> GPHMGAKWHLGIRSQSKPNDIMLEVYRAMKALSYEWKIINPYHVRVRRQNVKTGKFSKMSLQLYQVDAKSYLLDFKSLTNDEVEQGDDVIMESLTPPPLSVSGVMPLQPTGHHTMEFFEMCAALIIQLAR;> MYHQEPYISKPEERFKAPPILPPHLLQVILNKDTGISCDPALLPEPNHVMLNHLYALSIKDGVMVLSATHRYKKKYVTTLLYKPI;> MESVAAESAPAPENEHSQETPESNSSVYTTFMKSHRCYDLIPTSSKLVVFDTSLQVKKAFFALVTNGVRAAPLWDSKKQSFVGMLTITDFINILHRYYKSALVQIYELEEHKIETWREVYLQDSFKPLVCISPNASLFDAVSSLIRNKIHRLPVIDPESGNTLYILTHKRILKFLKLFITEFPKPEFMSKSLEELQIGTYANIAMVRTTTPVYVALGIFVQHRVSALPVVDEKGRVVDIYSKFDVINLAAEKTYNNLDVSVTKALQHRSHYFEGVLKCYLHETLEAIINRLVEAEVHRLVVVDEH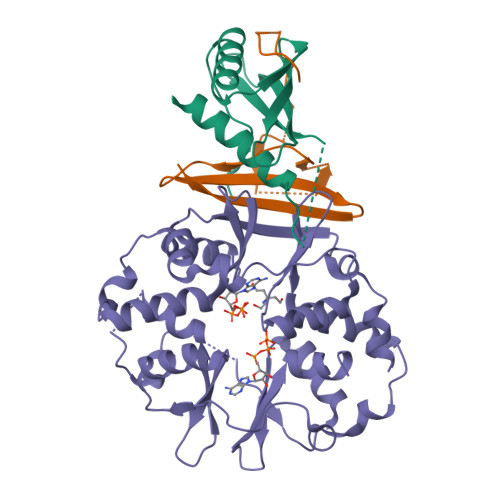DVVKGIVSLSDILQALVLTGGEKKP>[2x]GPLKPMTFSIYEGQEPSQIIFQFKANPPAVTFELTGETDNIFVIEREGLLYYNRALDRETRSTHNLQVAALDANGIIVEGPVPITIKVKDINDNRPTFLQSKYEGSVRQNSRPGKPFLYVNATDLDDPATPNGQLYYQIVIQLPMINNVMYFQINNKTGAISLTREGSQELNPAKNPSYNLVISVKDMGGQSENSFSDTTSVDIIVTE

Liver intestine (LI)-cadherin is a member of the cadherin superfamily, which encompasses a group of Ca2+-dependent cell-adhesion proteins. Human liver intestine–cadherin (LI-cadherin) is a nonclassical cadherin composed of an ectodomain consisting of seven extracellular cadherin (EC) repeats, a single transmembrane domain, and a short cytoplasmic domain. Because human LI-cadherin is expressed on gastric cancer cells but not on normal stomach tissues, LI-cadherin has been proposed as a target for imaging metastatic gastric cancer. Previous studies have reported that LI-cadherin works as a calcium ion–dependent cell adhesion molecule as other cadherins do.

Contrary to the canonical Ca2+-bound linker, such as the linker between EC1 and EC2, the linker between EC2 and EC3 in LI-cadherin does not contain Ca2+. Generally, three calcium ions bound to the linker between each EC repeat confer rigidity to the structure. Another unique characteristic in the region surrounding the calcium-free linker was the existence of an α-helix at the bottom of EC2. To the best of our knowledge, this element at the bottom of the EC2 is not found in classical cadherins.>MRGSHHHHHHGSEYPERPVNMVVPFAAGGPTDNVARSLAESMRPTLGETVVVENKGGAGGTIGTTQVARAQPDGYSILLMHAGFSTAPSLYKNPGYEPYTSFEPIGLVVDVPMTIIARGDFPPNNIKELAEYVKKNADKISLANAGIGAASHLCGTMLVEALGVNLLTIPYKGTAPAMNDLLGKQVDLMCDQTTNTTQQITSGKVKAYAVTSLKRVPTLPDLPTMDESGYKGFEVGIWHGMWAPKGTPKPVVDKLVKSLQAGLADPKFQERMK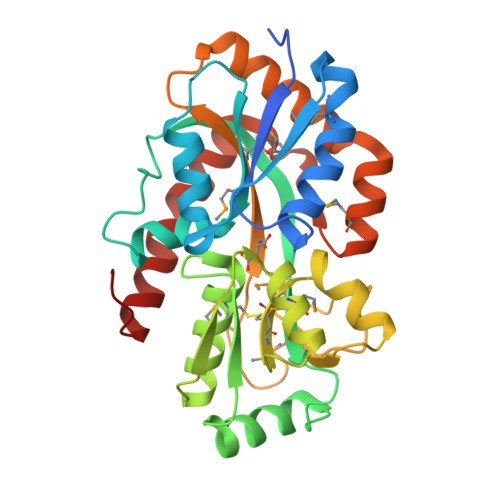QLGAEVLTNEANPEALQAKVKQQVPQWAELFKKAGVEKQ[3x]>GASGAPKLQPFTFPKTLHEGQTVKAICTPTEGERPLQFQWLKDGHPLMKRPLVDIK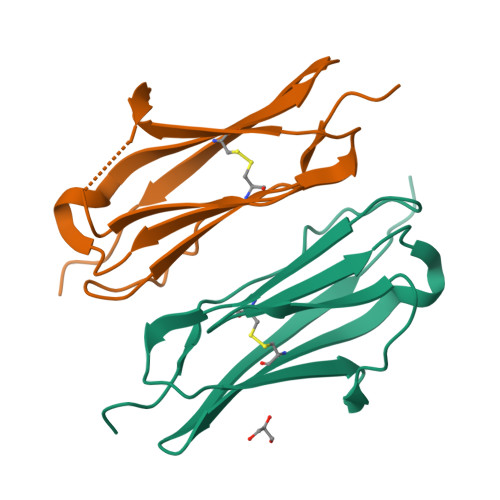TFEDYSLLKVSSVGEKDIGNYTCIVRNHHGSDQFTTSLTIPVA[2x]> TLNRLREPLLRRLSELLDQAPEGRGWRRLAELAGSRGRLRLSCLDLEQC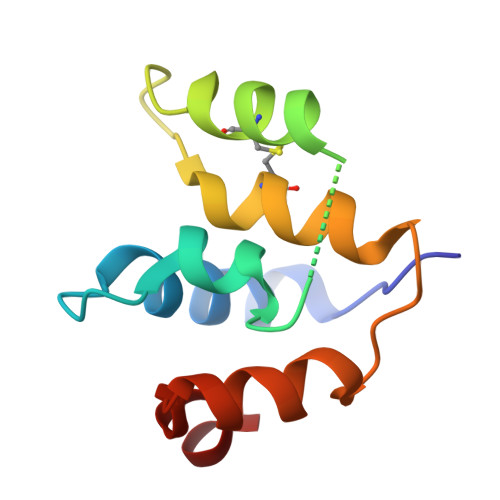SLKVLEPEGSPSLCLLKLMGEKGCTVTELSDFLQAMEHTEVLQLL> MEFSGRKWRKLRLAGDQRNASYPHCLQFYLQPPSENISLIEFENLAIDRVKLLKSVENLGVSYVKGTEQYQSKLESELRKLKFSYRENLEDEYEPRRRDHISHFILRLAYCQSEELRRWFIQQEMDLLRFRFSILPKDKIQDFLKDSQLQFEAISDEEKTLREQEIVASSPSLSGLKLGFESIYKIPFADALDLFRGRKVYLEDGFAYVPLKDIVAIILNEFRAKLSKALAL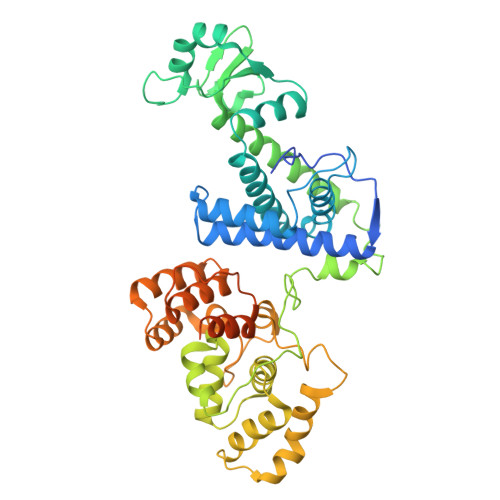TARSLPAVQSDERLQPLLNHLSHSYTGQDYSTQGNVGKISLDQIDLLSTKSFPPCMRQLHKALRENHHLRHGGRMQYGLFLKGIGLTLEQALQFWKQEFIKGKMDPDKFDKGYSYNIRHSFGKEGKRTDYTPFSCLKIILSNPPSQGDYHGCPFRHSDPELLKQKLQSYKISPGGISQILDLVKGTHYQVACQKYFEMIHNVDDCGFSLNHPNQFFCESQRILNGGKDIKKEPIQPETPQPKPSVQKTKDASSALASLNSSLEMDMEGLEDYFSEDS> APFVEDWDLVQTLGEGAYGEVQLAVNRVTEEAVAVKIVDMKRAVDCPENIKKEICINKMLNHENVVKFYGHRREGNIQYLFLEYCSGGELFDRIEPDIGMPEPDAQRFFHQLMAGVVYLHGIGITHRDIKPENLLLDERDN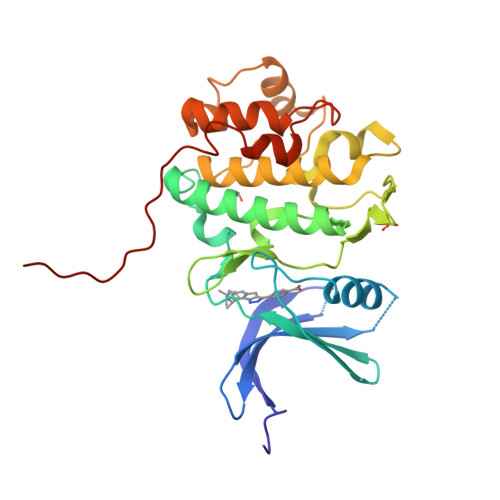LKISDFGLATVFRYNNRERLLNKMCGTLPYVAPELLKRREFHAEPVDVWSCGIVLTAMLAGELPWDQPSDSCQEYSDWKEKKTYLNPWKKIDSAPLALLHKILVENPSARITIPDIKKDRWYNKPLKKGAKRPRVTS5-PHOSPHOARABINONIC ACID | C5 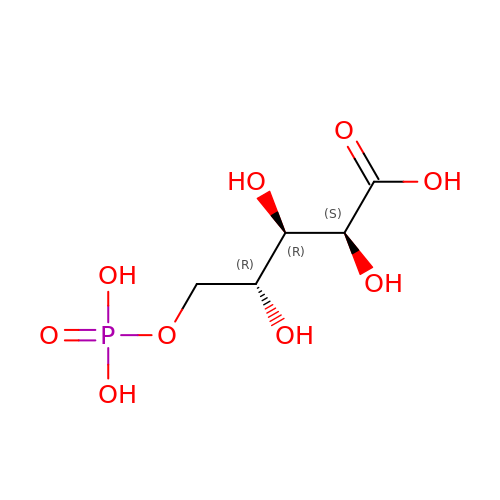H11 O9 P | HNECGPFIYSOYHF-JJYYJPOSSA-N4-[(1R,2S)-2-(carboxymethyl)cyclopentane-1-carbonyl]benzoic 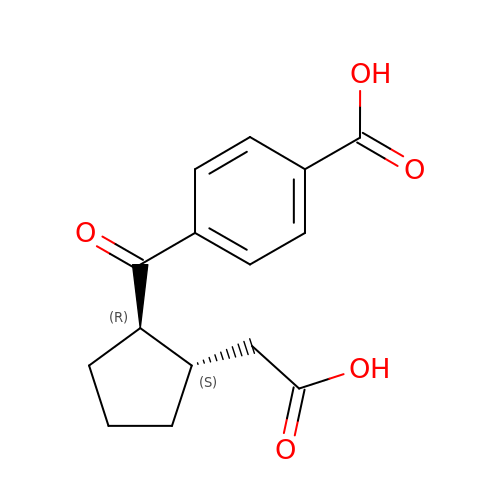acid | C15 H16 O5 | AIBKYDBZFDNIIN-NWDGAFQWSA-N> DVVVQAPTQVPGFLGDSVTLPCYLQVPNMEVTHVSQLTWARHGESGSMAVFH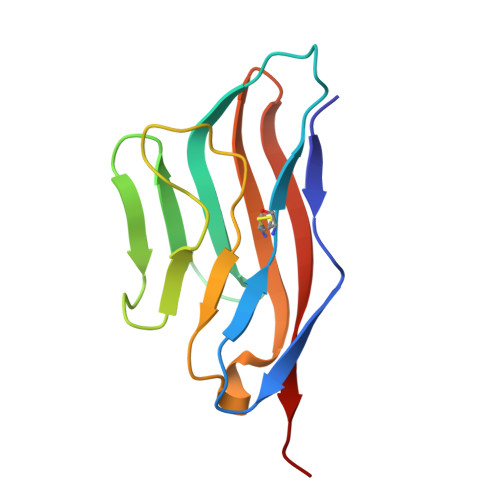QTQGPSYSESKRLEFVAARLGAELRNASLRMFGLRVEDEGNYTCLFVTFPQGSRSVDIWLRVLAKP(1S,2S,3S,4R,5R)-2-({[5-(hydroxymethyl)furan-2-yl]methyl}amino)-4-(morpholin-4-yl)-6,8-dioxabicyclo[3.2.1]octan-3-ol | C16 H24 N2 O6 | 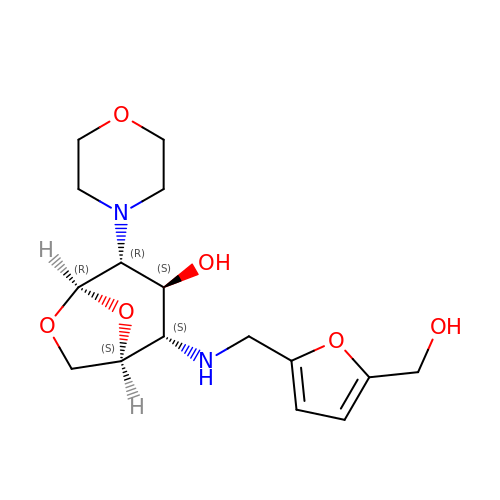QPKSUNGYGHKTGL-DGXTUMSLSA-N>[2x]GPHMPA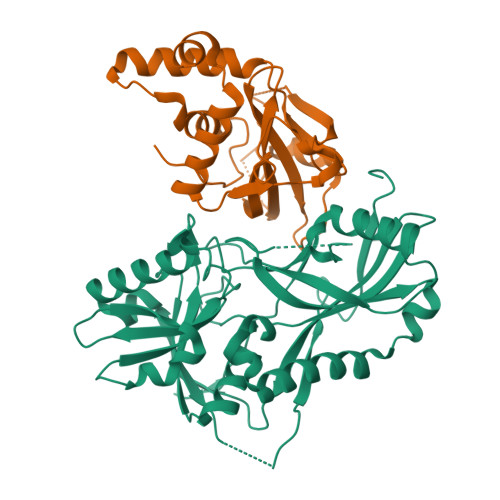IILQFAPLNSSVDEGFWHSFSSLKLDKLGIDDSPISITGFYGPCGHPQVSNHLTLLSESLPLDEQSLIASTSHGNRNKCPVPGILYNTNTVESFNKLDKQSLLKAEANKIWEDIQSGKALEDPSVLPRFLVISFADLKKWSFRYWFAFPAFVLDPPVSLIELKPASEYFSSEEAESVSAACNDWRDSDLTTDVPFFLVSVSSDSKASIRHLKDLEACQGDHQKLLFGFYDPCHLPSNPGWPLRNYLALIRSRWNLETVWFFCYRESRGFADLNLSLVGQASITLSSGESAETVPNSVGWELNKGKRVPRSISLANSM;>GPHMAFKEKGVLSVSEFVLAGDNLVSKCPTWSWESGDASKRKPYLPSDKQFLITRNVPCLRRAASVAEDYEAAGGEVLVDDEDNDGWLATHGKPKDKGKEEDNLPSMDALDINEKNTIQSIPTYFGGEEDDDIPDMEEFDEADNVVENDPATLQSTYLVAHEPDDDNILRTRTYDLSITYDKYYQTPRVWLTGYDESRMLLQPELVMEDVSQDHARKTVTIEDHPHLPGKHASVHPCRHGAVMKKIIDVLMSRGVEPEVDKYLFLFLKFMASVIPTIEYDYTMDFDLGSSST[2x]>MSVTGTEIDSDTAKNILSVDELQNYGINASDLQKLKSGGIYTVNTVLSTTRRHLCKIKGLSEVKVEK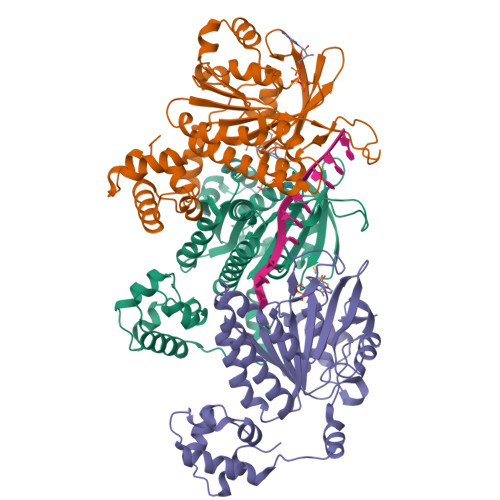IKEAAGKIIQVGFIPATVQLDIRQRVYSLSTGSKQLDSILGGGIMTMSITEVFGEFRCGKTQMSHTLCVTTQLPREMGGGEGKVAYIDTEGTFRPERIKQIAEGYELDPESCLANVSYARALNSEHQMELVEQLGEELSSGDYRLIVVDSIMANFRVDYCGRGELSERQQKLNQHLFKLNRLAEEFNVAVFLTNQVQSDPGASALFASADGRKPIGGHVLAHASATRILLRKGRGDERVAKLQDSPDMPEKECVYVIGEKGITDSSD[3x]> MGCTYTIQPGDT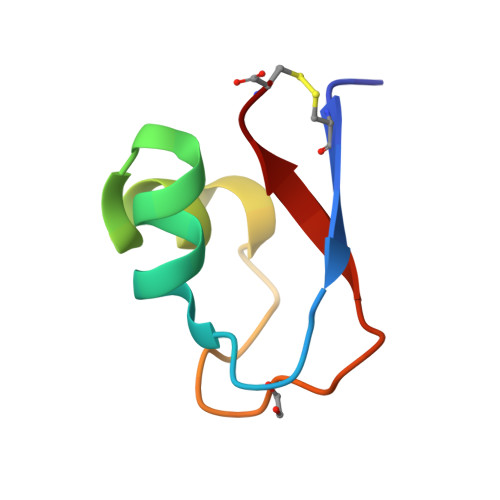FWAIAQRRGTTVDVIQSLNPGVNPARLQVGQVINVPC> AMAISDPQSSTRNELETGSSSACPKVIYIFARASTEPGNMGISAGPIVADALERIYGANDVWVQGVGGPYLADLASNFLPDGTSSAAINEARRLFTLANTKCPNAAIVSGGYSQGTAVMAGSISGLSTTIKNQIKGVVLFGYTKNLQNLGRIPNFETSKTEVYCDIADAVCYGTLFILPAHFLYQT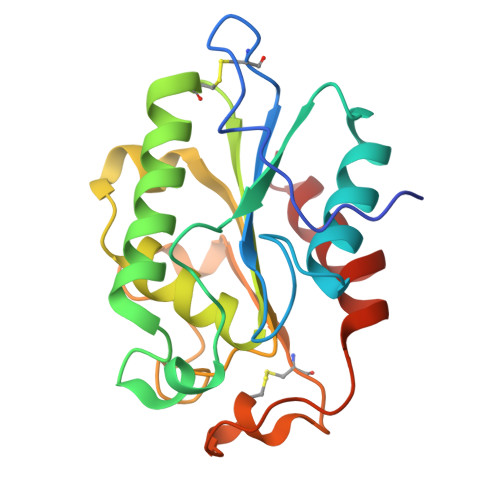DAAVAAPRFLQARIG>ITSSKFNECQLNNLNALEPDHRVESEGGLIETWNSQHPELQCAGVTVSKRTLNRNGLHLPSYSPYPQMIIVVQGKGAIGFAFPGCPETFEKPQQQSSRRGSRSQQQLQDSHQKIRHFNEGDVLVIPPGVPYWTYNTGDEPVVAISLLDTSNFNNQLDQNPRVFYLAGNPDIEHPETMQQQQQQKSHGGRKQGQHQQQEEEGGSVLSGFSKHFLAQSFNTNEDTAEKLRSPDDERKQIVTVEGGLSVISPKWQEQEDEDEDEDEEYEQTPSYPPRRPSHGKHEDDEDEDEEEDQPRPDHPPQRPSRPEQQEPRGRGCQTRNGVEENICTMKLHENIARPSRADFYNPKAGRISTLNSLTLPALRQFGLSAQYVVLYRNGIYSPHWNLNANSVIYVTRGKGRVRVVNCQGNAVFDGELRRGQLLVVPQNFVVAEQGGEQGLEYVVFKTHHNAVSSYIKDV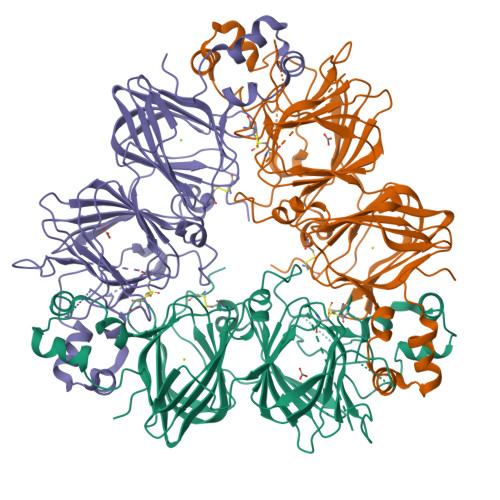FRAIPSEVLSNSYNLGQSQVRQLKYQGNSGPLVNP[6x]>[8x]MEGISIYTSDNYTEEMGSGDYDSMKEPCFREENANFNKIFLPTIYSIIFLTGIVGNGLVILVMGYQKKLRSMTDKYRLHLSVADLLFVITLPFWAVDAVANWYFGNFLCKAVHVIYTVNLYSSVLILAFISLDRYLAIVHATNSQRPRKLLAEKVVYVGVWIPALL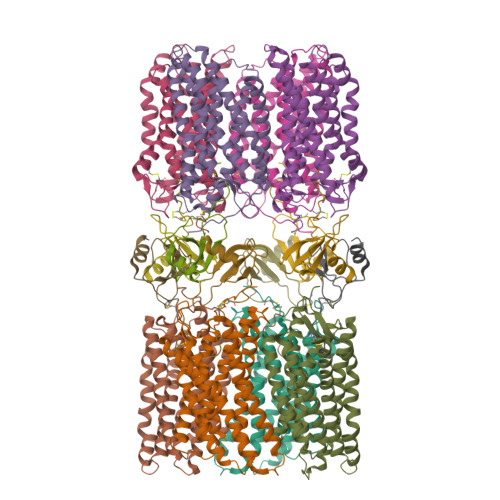LTIPDFIFANVSEADDRYICDRFYPNDLWVVVFQFQHIMVGLILPGIVILSCYCIIISKLSHSKGHQKRKALKTTVILILAFFACWLPYYIGISIDSFILLEIIKQGCEFENTVHKWISITEALAFFHCCLNPILYAFLGAKFKTSAQHALTSVSRGSSLKILSKGKRGGHSSVSTESESSSFHSSDYKDDDDK;>[8x]KPVSLSYRCPCRFFESHVARANVKHLKILNTPNCALQIVARLKNNNRQVCIDPKLKWIQEYLEKALNKRFKMHHHHHHHH4-carbamimidamidobutanoic 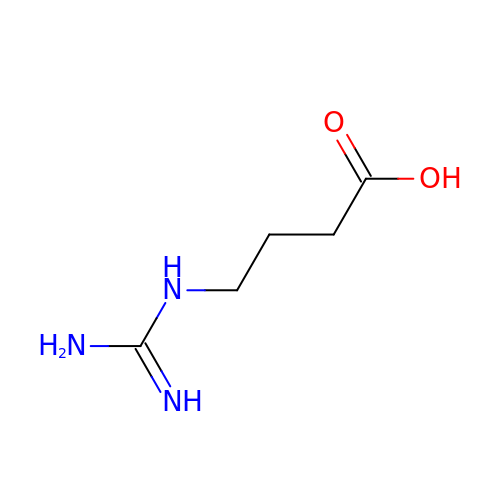acid | C5 H11 N3 O2 | TUHVEAJXIMEOSA-UHFFFAOYSA-N>ETIASELKAIGKELEDQKKEENIQIAKIAKEKFDFLSTFKVGPYDLIDEDIQMKIKRTLYSSLDYKKENIEKLKEILEILKKNSEHYNIIGRLIYHISWGIQFQIEQNLELIQNGVENLSQEESKSLLMQIKSNLEIKQRLKKTLNETLKVYNQNTQDNEKILAEHFNKYYKDFDTLKPAF[4x]

CspA (also referred to as BbCRASP-1 or BBA68) is expressed on the surface of B. burgdorferi and binds factor H and FHL-1 in the region of domains 5–7 with an affinity measured in the range 10–30 nM. The atomic structure of CspA is known and consists of seven α-helices joined by short loops assembled in a ‘lollipop’-type arrangement. The crystal structure shows the formation of a homodimeric species mediated by inter­actions between helix F in both subunits. The dimeric structure possesses a cleft between the two subunits within which a putative factor H binding site has been proposed following in vitro mutagenesis studies.

The structure of CspA from B. burgdorferi has been redetermined to 4.1 Å resolution in a new crystal form, showing that the bacterial protein exists in a dimeric form which is highly similar to that observed in the previous crystal structure. Presented here is a new crystal structure of CspA showing a different conformation between the dimer subunits, demonstrating a degree of flexibility which has implications for the accessibility and conformation of the binding site. The differences between the two CspA structures are likely to arise from the different crystal packings. However, these structures illustrate that flexibility between the subunits is mediated by distortion of helix F between residues 225 and 227. This leaves the structure of the ten C-terminal residues (240–250) unaffected, supporting earlier evidence that these residues are required for the assembly of a stable dimer. Further weight is also added to the hypothesis that the dimeric species is essential for the function of CspA as the ‘lock’ to the second subunit is unaffected. Despite flexibility in the dimer organization, the C-terminal lock structure is completely conserved, suggesting that these interactions underpin the assembly and therefore the biological activity of CspA. Flexibility also allows alteration of the binding-site confirmation which could enable binding to different complement regulators, perhaps providing a key role of CspA in enabling B. burgdorferi to evade complement-mediated killing.>MKKLKVMTVFGTRPEAIKMAPLVLELKKYPEIDSYVTVTAQHRQMLDQVLDAFHIKPDFDLNIMKERQTLAEITSNALVRLDELFKDIKPDIVLVHGDTTTTFAGSLAAFYHQIAVGHVEAGLRTGNKYSPFPE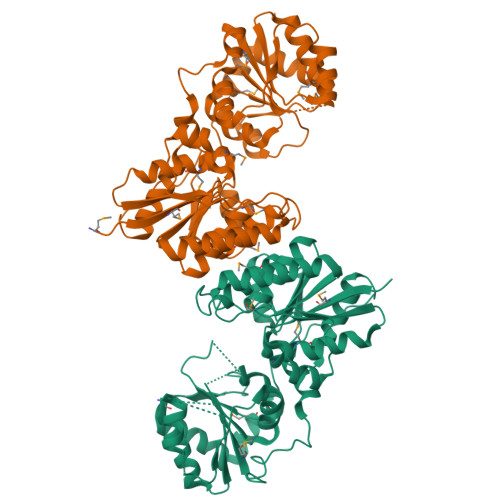ELNRQMTGAIADLHFAPTGQAKDNLLKENKKADSIFVTGNTAIDALNTTVRDGYSHPVLDQVGEDKMILLTAHRRENLGEPMENMFKAIRRIVGEFEDVQVVYPVHLNPVVREAAHKHFGDSDRVHLIEPLEVIDFHNFAAKSHFILTDSGGVQEEAPSLGKPVLVLRDTTERPEGVEAGTLKLAGTDEENIYQLAKQLLTDPDEYKKMSQASNPYGDGEASRRIVEELLFHYGYRKEQPDSFTGKGSHHHHHH[2x]>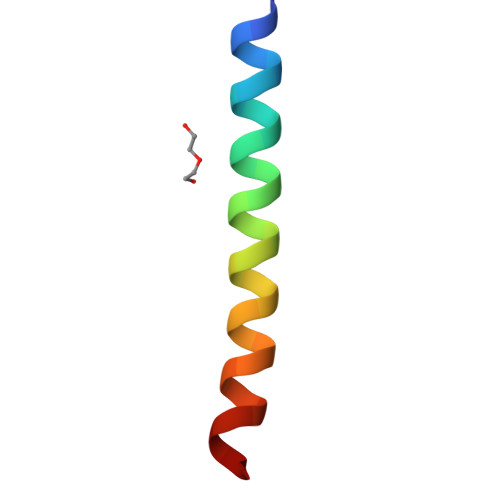[2x]SAASDLDELLWVIAVTIFGLVLIASILKFYK DapF (EC 5.1.1.7), a pyridoxal 5-phosphate-independent amino acid racemase, catalyzes the stereochemical inversion between l,l-DAP and d,l-DAP. DapF plays an important role in the biosynthesis of l-lysine because DAP decarboxylase only recognizes d,l-DAP. Each CgDapF monomer consists of two distinct domains: an N-terminal domain (NTD; Met1–Asp131 & Gly268–Ile277) and a C-terminal domain (CTD; Met132–Thr267). Two catalytic cysteine residues are positioned at the active site, which is located at a cleft between the two domains.

To reveal the molecular mechanism of CgDapF, we determined its crystal structure (2.0 Å resolution) via the single-wavelength anomalous dispersion method, using a selenium-substituted crystal. In one monomer, two catalytic cysteine residues (Cys83 and Cys221) were oxidized, forming a disulfide bond with each other; in contrast, these residues were reduced in the other monomer. The formation of this disulfide bond also caused a large conformational change in the loop that contains Cys83 (Ala75–Gly84). In contrast, in the oxidized form of CgDapF, the loop was positioned 5.8 Å closer to the substrate binding site, compared to the reduced form, resulting in closure of the substrate binding site. In contrast, in the oxidized form of CgDapF, the DC-loop interacts with the CTD instead. The disulfide bond between Cys83 and Cys221 is the main contributor to the stability of the loop, and the side chain of Thr223 forms hydrogen bonds with the main chain portions of Met82 and Cys83. In fact, no reducing agent was added, neither to the reservoir nor to the protein solution used for crystallization, indicating that the protein was crystallized under somewhat oxidized condition. In particular, the DC-loop of the oxidized monomer makes a close contact with one neighboring molecule, whereas that of the reduced monomer makes no contact with any molecule. Under oxidized condition, the position of the DC-loop occludes the active site, which inactivates the enzyme.

>MNLTIPFAKGHATENDFIIIPDEDARLDLTPEMVVTLCDRRAGIGADGILRVVKAADVEGSTVDPSLWFMDYRNADGSLAEMCGNGVRLFAHWLYSRGLVDNTSFDIGTRAGVRHVDILQADQHSAQVRVDMGIPDVTGLSTCDINGQVFAGLGVDMGNPHLACVVPGLSASALADMELRAPTFDQEFFPHGVNVEIVTELEDDAVSMRVWERGVGETRSCGTGTVAAACAALADAGLGEGTVKVCVPGGEVEVQIFDDGSTLTGPSAIIALGEVQIHHHHHH[2x]> SAKGIDYDKLIVRFGSSKIDKELINRIERATGQRPHHFLRRGIFFSHRDMNQVLDAYENKKPFYLYTGRGPSSEAMHVGHLIPFIFTKWLQDVFNVPLVIQMTDDEKYLWKDLTLDQAYSYAVENAKDIIACGFDINKTFIFSDLDYMGMSSGFYKNVVKIQKHVTFNQVKGIFGFTDSDCIGKISFPAIQAAPSFSNSFPQIFRDRTDIQCLIPCAIDQDPYFRMTRDVAPRIGYPKPALLHSTFFPALQGAQTKMSASDPNSSIFLTDTAKQIKTKVNKHAFSGGRDTIEEHRQFGGNCDVDVSFMYLTFFLEDDDKLEQIRKDYTSGAMLTG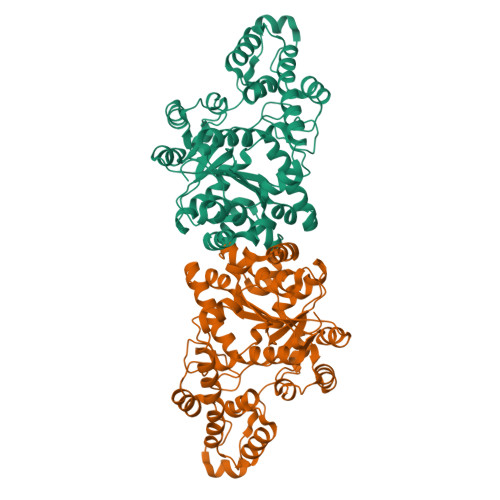ELKKALIEVLQPLIAEHQARRKEVTDEIVKEFMTPRKLSFDFQ>HMTIPGRFMTIDKGTFGEYTASTRWPIIIQNAIDDLSKHQETEKSNGTKFEQGEVIKKELKEFRQEIIDRVPLRPFTEEEIKIANVPLSFNEYLKKHPEVNWGAVEWLFSEVYLYRRVNVLFQRQCEWAKFDIFNRLKQSTFESSFYGVVELALRYENLLPQLREMKQNPGNEIDDILKVLFKEFIEISLWGNATDLSLLTNATLEDIKSIQGAKARAASESKIVVNDTEKAWEVLTKARADANSREIRVDFVLDNSGFELYADLMLAAFLLQSGLATKCIFHAKDIPYMVSDVMLKDFDILVHDLRDREFFPSGEPSTKESRALDLFAGEMEKFVSSGKIEFREDSFWTTELDYWNLDANETKYHGSILHKDLQKSNLVI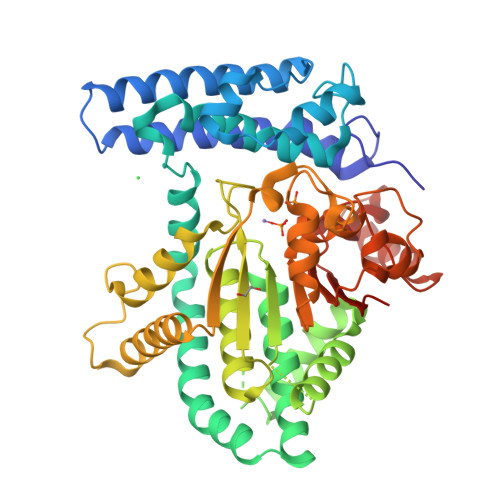FKGDLNYRKLTGDRKWPRTTKWETAIGPLATNGITSLSLRTCKADVQVALPEGLDAKLSQEWEKENPGRGSWWCCSGKWAVICFCSGIHK[3x]>[4x]ADSDVPNDILEEQLYNSIVVADYDSAVEKSKHLYEEKKSEVITNVVNKLIRNNKMNCMEYAYQLW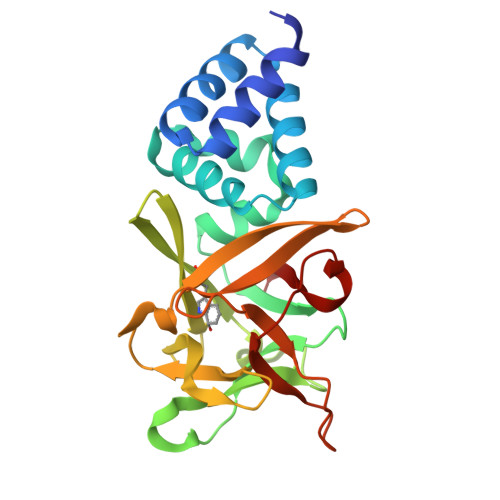LQGSKDIVRDCFPVEFRLIFAENAIKLMYKRDGLALTLSNDVHGNDGRLAFGDGKDKTSPKVSWKFIALWENNKVYFKILNTERNQYLVLGVGTNPNGDHMAFGVNSVDSFRAQWYLQPAKYDKDNLFYIYNREYSKALTLSRTLETSGNRMAWGYNGRVIGSPEHYAWGVKAF N-({6-[(4-CYANO-2-FLUOROBENZYL)OXY]NAPHTHALEN-2-YL}SULFONYL)-D-GLUTAMIC ACID | C23 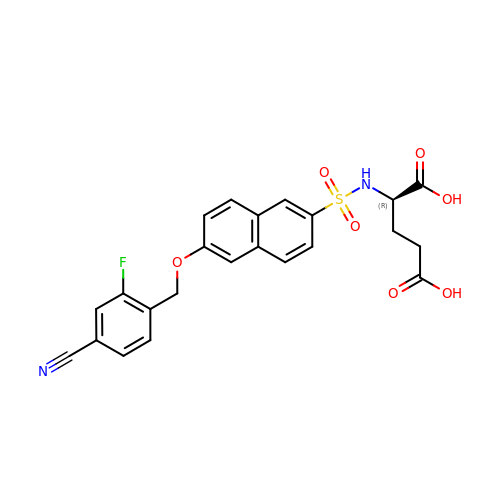H19 F N2 O7 S | IRJUSGUHNFMVCK-OAQYLSRUSA-N2-methoxycarbonylbenzoic acid 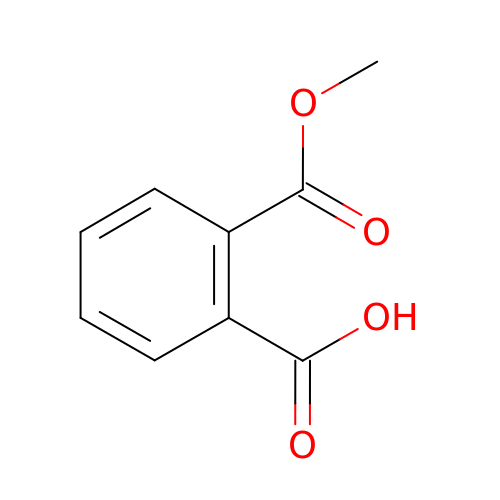| C9 H8 O4 | FNJSWIPFHMKRAT-UHFFFAOYSA-N> MRGSHHHHHHGSMPFEIVFEGAKEFAQLIETASRLIDEAAFKVTEEGISMRAMDPSRVVLIDLNLPASIFSKYEVDGEETIGVNMDHLKKVLKRGKAKETLILRKGEENFLEISLQGTATRTFKLPLIDVEEIEVDLPELPFTAKVVILGDVIKEAVKDASLVSDSMKFIAKENEFTMRAEGETQEVEVKLTLEDEGLLDIEVQEETKSAYGISYLSDMVKGLGKADEVTIKFGNEMPMQMEYYIRDEGRLIFLLAPRVEE;> KKRVISLEEFFS

The bacterial sliding clamp is referred to as the β clamp, whereas the eukaryotic and archaeal sliding clamp protein is called the proliferative cell nuclear antigen (PCNA). Clamps are constructed from either two (β) or three monomers (PCNA) to yield a ring composed of six domains, which share similar protein folds. Hence, across every domain of life, the extraordinary efficacy of the replicative polymerase complex is dependent on their interaction with sliding clamps, which encircle DNA and greatly enhance their processivity. We have shown that PolD uses two distinct PIP-boxes for molecular recognition of PCNA, which are located in the C-terminal region of their DP2 subunit.

To better characterize the role of cPIP, we co-crystallized PCNA from P. abyssi with a 12 amino-acid peptide mimicking the DP2 cPIP and solved its structure at 2.7 Å resolution. The final model includes 9 of the 12 amino acids of the co-crystallized peptide. In contrast to the structure of iPIP, which differs from other structures of PIP-boxes, cPIP shares the same overall fold as those described in the literature. Hence, the cPIP structure shows an extended peptide chain, whose C-terminal region folds into a 310 helix. Several conserved hydrophobic residues of the cPIP—V1258, I1259, L1261, and F1264—insert their bulky side chains into the hydrophobic cleft formed by the PIP-binding pocket on the PCNA surface. It is noteworthy that cPIP lacks the consensus Q residue, which is present in most PIP-boxes. The cryo-EM and crystal structures reveal that cPIP and iPIP adopt redundant binding positions in the PCNA PIP-binding pocket. Indeed, the side chains of L1199 and L1201 in iPIP and the side chains of I1259 and L1261 in cPIP are accommodated similarly in the PCNA-binding pocket, suggesting that the binding of iPIP and cPIP to PCNA are mutually exclusive. The cPIP binds to PCNA with a lower affinity (KD of 49 ± 4 μM), which differs by two orders of magnitude from the one observed for the MBP–iPIP–cPIP fusion, suggesting that the flanking region may be important for binding to PCNA. Deleting cPIP in the MBP–iPIP-ΔcPIP fusion (DP2:1196–1253) strongly impaired binding to PCNA and abrogated binding to the DNA primase, showing that cPIP is a dual PCNA/primase-binding peptide.> GPGSNCGPPPTLSFAAPMDITLTETRFKTGTTLKYTCLPGYVRSHSTQTLTCNSDGEWVYNTFCIYKRCRHPGELRNGQVEIKTDLSFGSQIEFSCSEGFFLIGSTTSRCEVQDRGVGWSHPLPQ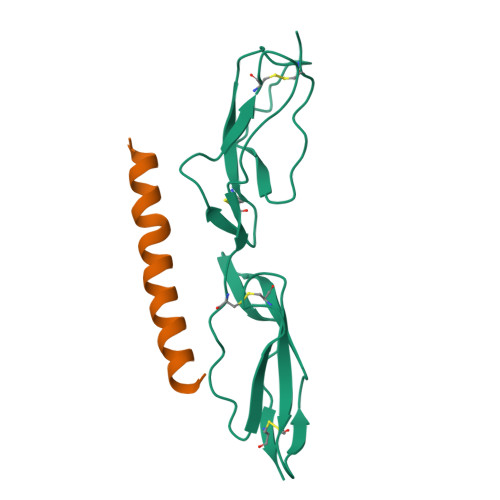CEI;> GPGSAESPKSTETSANGADKLADAYNTLLTEHEKLRDEYYTLIDAKEEEPRYKALRGENQDLREKEGKYQDKIKKLEEKEKNLEKKSEDVERHYLKKLDQEHKE> GSMAPRAGFDAEQVRDKARKDLLHLLEGVRGKKNLVIEKDLAGPLGVIVKASTLRDYGVDNFFFLENKNTGTSQRNIVFIARGESVRNAHAIAAQIKRIQRESQTSHDFHIFWVPRRTLFSDKVLEEAGVLGDANISELPLYFFPLERDVLSLELNDSFRDLYLAKDPTPVFLLSRALMGIQKKHGLFPRIIGKGENAKRVADLLSRMRQELLAGEEAGESDRAGLSPSTTIESVIIIDREVDFVTPLLTQLTYEGLIDEYFGIQNNQTDVDAVIVGAPAQSAASTSTAVPTNSSQSRKRKIQLDGSDSLYSQLRDANFAIVGSLLNTVARRLKSDYESRHNTKTTAELKEFVKKLPGYQAEQQSLKIHSNIAEEIINYTRTEIFNKLLEVQQNLAAGADPSSQFDSIEELVARDTPLPQVLRLLCLYSCISGGIKTKELDHFRRLVLQGYGHQHLLTLHNLERLQMFLSKSSPLASMITMSGSSGGPDQKTNYTYLRKQLRLIVDEVNEQDPNDIAYVYSGYAPLSIRLVQCVLQKQYLLSITKGSGTVIAAGPVAGGGAQGWKGFEEIVKHARGPTFDEIQKGEDKAVKARALLSGSSGDKKTVFVVFVGGITFTEIAALRFIAKQEEARRNIVICTTSIINGNRMMNAAIETATFEKTTVTTAAAQ;> MGSSFEVIARTAYEEGRTRLATELLNHEPRAGRQVPLLLSMEEDELALDKAIESGDTDLIYFVIHQLRRKLPLASFFRVVSSRPTASAMVEA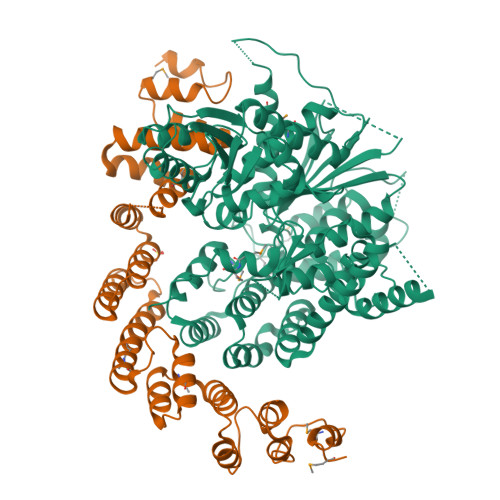LARNSDGDGNEDTALLKDLYYQDDRRLDGASVFIREALQQPETRTASDKLDLAANLLQGNQKEHVFELGALKEAKMLLRMQETFERDLTDSFVGLSVNQTMFKLIKLGYHGRAKKIQSEFKVPERVAWWIRLQALVAKRDWNEIEEISRQRKSPIGWEPFFNQVLQAGNPRLAATFIPKCTNLEPGQTITMYEKCGMRVKAAEEAVRLKDTEAWNRLLEAAGRNTAEGREIERLGATVFKK>MKLSKDTIAILKNFASINSGILLSQGKFIMTRAVNGTTYAEANISDEIDFDVALYDLNSFLSILSLVSDDAEISMHTDGNIKIADTRSTVYWPAADKST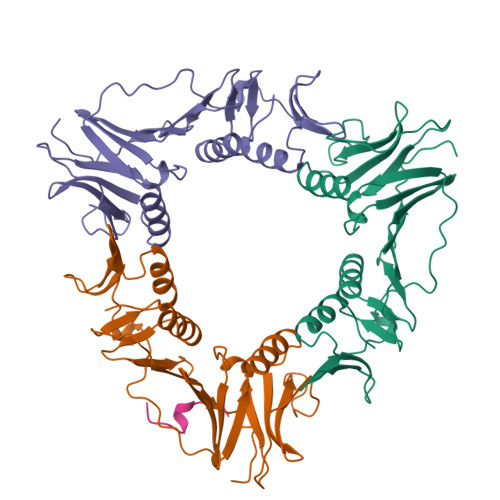IVFPNKPIQFPVASVITEIKAEDLQQLLRVSRGLQIDTIAITNKDGKIVINGYNKVEDSGLTRPKYSLTLTDYDGSNNFNFVINMANMKIQPGNYKVMLWGAGDKVAAKFESSQVSYVIAMEADSTHDF[3x];> KKASLFDMFDF> GPLSMSCWLREQTLLLAE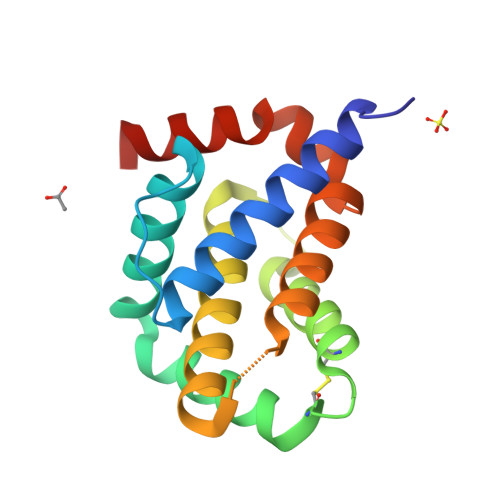DYISFCSGIQQTPPSESAEAMRYLAKEMEQQHRTKFRSLSQEFLDTCGADPSKCLQSVMRELVGDGKMNWGRVVSIFTFTGVLASELLSRGENSEGSRRLAETIADYLGGEKQDWLVENGGWEGFCRFFHNARQ>[2x]MKVWNARNDHLTINQWATRIDEILEAPDGGEVIYNVDENDPREYDAIFIGGGAAGRFGSAYLRAMGGRQLIVDRWPFLGGSCPHNACVPHHLFSDCAAELMLARTFSGQYWFPDMTEKVVGIKEVVDLFRAGRNGPHGIMNFQSKEQLNLEYILNCPAKVIDNHTVEAAGKVFKAKNLILAVGAGPGTLDVPGVNAKGVFDHATLVEELDYEPGSTVVVVGGSKTAVEYGCFFNATGRRTVMLVRTEPLKLIKDNETRAYVLDRMKEQGMEIISGSNVTRIEEDANGRVQAVVAMTPNGEMRIETDFVFLGLGEQPRSAELAKILGLDLGPKGEVLVNEYLQTSVPNVYAVGDLIGGPMEMFKARKSGCYAARNVMGEKISYTPKNYPDFLHTHYEVSFLGMGEEEARAAGHEIVTIKMPPDTENGLNVALPASDRTMLYAFGKGTAHMSGFQKIVIDAKTRKV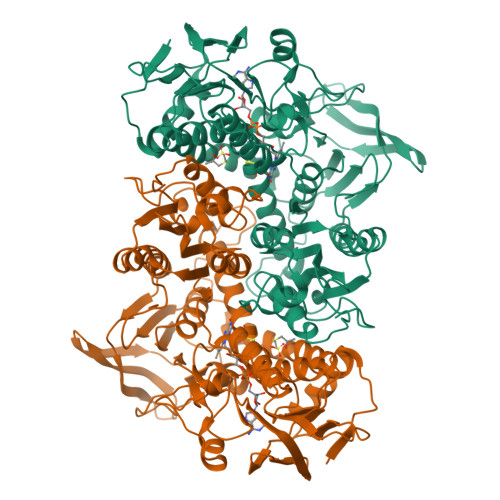LGAHHVGYGAKDAFQYLNVLIKQGLTVDELGDMDELFLNPTHFIQLSRLRAGSKNLVSL>MESSKTEQVTGATGITQSTVTAPLPEAVSSLSLAPTVNALDPWVYLNQTEVPGGTFTVSSATQPGSVLLELEISPELNLYTSHLFRMYAGWSGGFSLKLLVAGNAFSAGKLIAAIIPPNIEVPNSAYLLTGFPHEILDFRTADSMEIIAPDIKNIDYHFRGDKLGKLVVMVYSPLRST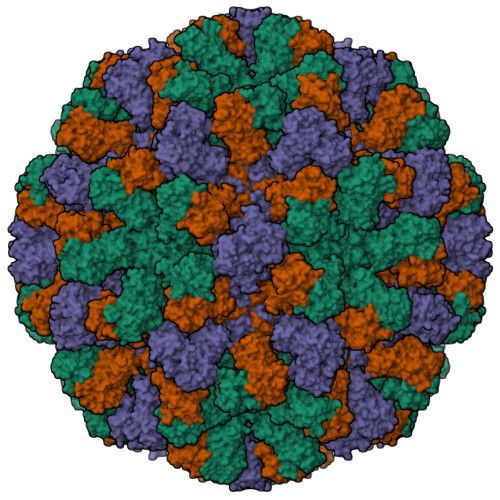SADFEIEIKLTSAPLPDFKFTMLVPPIQNNALPIWSIPQAPPYSMVNPRSPLTPVVELYINSSYATCNHQLGRYTIYQGAIGNSTFNPSGAWTATCTAEAGSVTGHPNWRYALLDLPDNPTFDPTLPPVPRGFCDWGSGVKSGNKQHLVCFTGKKVEGGFQDVDTHMWDYGDNETVGLDNTYQRTIYIKDPSLEKDAQYLVIPMGVSGAANDDTVQVAPNCYGSWDYAPTVAPPLGEQFVWFRSQLPASKTTTTSGVNSVPVNVNALMSPDLMCSAYASGFPLGKVALLDYVLFGGSVVRQFKLYPEGYMTANTTGSNTGFIIPADGYFRFNSWVSPSFMISSVVDLNLQTAVVFR[3x]>[2x]ACGLVASNLNLKPGECLRVRGEVAADAKSFLLNLGKDDNNLCLHFNPRFNAHGDVNTIVCNSKDAGAWGAEQRESAFPFQPGSVVEVCISFNQTDLTIKLPDGYEFKFPNRLNLEAINYL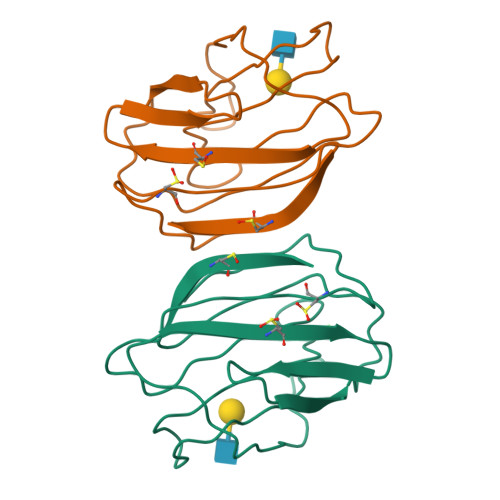SAGGDFKIKCVAFE> MLEEIMKYEASILTHDSSIRYLQEIYNSNNQKIVNLKEKVAQLEAQCQEPCKDTVQIHDITGKDCQDIANKGAKQSGLYFIKPLKANQQFLVYCEIDGSGNGWTVFQKRLDGSVDFKKNWIQYKEGFGHLSPTGTTEFWLGNEKIHLISTQSAIPYALRVELEDWNGRTSTADYAMFKVGPEADKYRLTYAYFAGGDAGDAFDGFDFGDDPSDKFFTSHNGMQFSTWDNDNDKFEGNCAEQDGSGWWMNKCHAGHLNGVYYQGGTYSKASTPNGYDNGIIWATWKTRWYSMKKTTMKIIPFNRLTIGEGQQH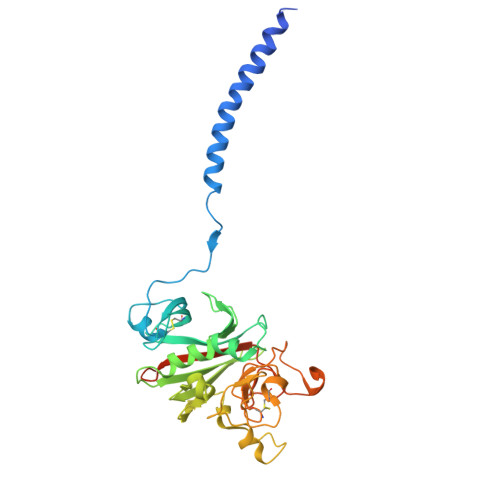HLGGAKQAGDV> GNNDDDGTNKAQEIAGKYEGYSIGNCAMFTDYVMGEKSVATIVPNEDGTINVTYDSGSGEFKLNNIKVTSKTFEGSGQVELSMNDKPAGAKDFTLTGSIDEQQKLTLKVNVPSVMGGLTIEFIQGTLPISYHVSGTYNKEANLSVSVGSTTYPDITDCKVSIKRSSDDTVELTLKGLSNLNSSQTGRAMNLGDFTVTDVKVTSTDN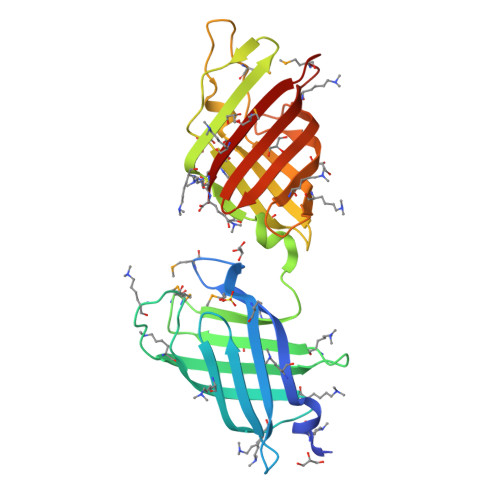SIFKIEGSINTTDTNNTPITGTLSGTVSNSETNITFTFKPGAMPIDITAMFKGKK To confer the favorable attributes of ABEs upon a CBE, we envisioned transforming TadA into an enzyme capable of robust cytidine deamination and subsequently generated an improved class of CBEs that uses TadA instead of a naturally occurring cytidine deaminase. Here we describe the development of two families of base editors, CABE-Ts and CBE-Ts, which use variants of TadA to catalyze the deamination of cytosines with either retention (CABE-Ts) or loss (CBE-Ts) of adenine deamination. To illuminate how amino acid substitutions identified from directed evolution affect TADAC’s substrate tolerance, we determined crystal structures of TadA*8.20 from ABE8.20-m13, the template used to evolve CABE-T1, and TADAC-1 variants from CABE-T1 reported here. Through X-ray crystallography, we show how the accumulation of substitutions impacts the shape of the active site cavity and may contribute to the accommodation of cytosine as substrate and the subsequent shift in specificity toward C-to-U deamination.

Crystal structures of TadA*8.20 and TADAC-1.17 were determined in a complex with ssDNA substrate containing the adenine transition-state analog 2-deoxy-8-azanebularine (d8Az). These two structures are highly similar, and the four TADAC-1.17 substitutions (T17A, A48G, S82T and A142E) derived from evolution do not drastically alter substrate tolerance by changing the protein structure or the ssDNA binding mode.

>[4x]MSEVEFSHEYWMRHALTLAKRARDEREVPVGAVLVLNNRVIGEGWNRAIGLHDPTAHAEIMALRQGGLVMQNYRLYDATLYSTFEPCVMCAGAMIHSRIGRVVFGVRNAKTGAAGSLMDVLHHPGMNHRVEITEGILADECAALLCRFFRMPRRVFNAQKKAQSSTD>GSHMMDARIVNALIGSVYETIRDVLGIEPKTGKPSTVSHIEIPHSLVTVIGITGGIEGSLIYSFSSETALKVVSAMMGGMEYNQLDELALSAIGELGNMTAGKLAMKLEHLGKHVDITPPTVVSGRDLKIKSFGVILKLPISVFSE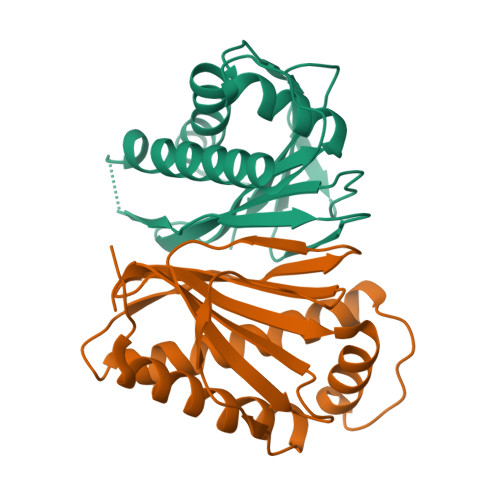EDFDLHLSVKSGG[2x]> MEELFNALPQPLQQLSLALAGEIPLTDHIFEQAASTWHVQPRSLTYKLLDHIPFATPVVVPPSIYHSLDWSKCFAVNQDRVERIPTIDNPDDVYVPNSDIGPLLTSLHTIPDYGFLHPTIENDATTLRAERARCASTFYKIASSQARQVKLDPIRMLGFLLLVQARPRVPSGLVTDQPTRRDPTLSPALHAIWQVMQYYKVAGVYYAPALVVPSGAIWWIPPPGKRNVVSVQYLLTDLISLAILAHMTDMSPTLELTGVLMYLRAASSHSYAYTLLQMKSVFPALSLRSMYRNKGFGGKAPAIEWTEPRSKYKFRWTGVTQLHDGLRPRSPSMDVPTLETLAKYELVDIGHTIIRERNAHPQHNHDSVRFVRDVMALTSGMYLVRQPTMSVLREYSQVPDIKDPIPPSAWTGPIGNVRYLLPSVQGPARHLYDTWRAAARQIAQDPQWHDPLNQAIMRAQYVTARGGSSASLKFALKVTGIVLPEYDDSKVKKSSKIYQAAQIARIAFMLLIAAIHAEVTMGIRNQVQRRARSIMPLNVIQQAISAPHTLVANYINKHMNLSTTSGSVVTDKVIPLILYASTPPNTVVNVDIKACDASITYNYFLSVICGAMHEGFEVGNADAAFMGVPSTIVSDRRSPVAPYSRPISGLQTMVQHLADLYAAGFRYSVSDAFSSGNKFSFPTSTFPSGSTATSTEHTANNSTMMEYFLNVHAPSHVKSASLKRILTDMTIQRNYVCQGDDGILLLPHEAASKISADDMNELLTCLRDYGQLFGWNYDIDWSDTAEYLKLYALMGCRIPNTSRHPPVGKEYAAPQTDEIWPSLIDIVIGHHLNGVTDVLNWREWLRFSWAFACYSSRGGYTNPRGQSFSAQYPWWTFVYLGIPPILLPGQTPFIHSCYMPPGDQGMFSILNGWRDWLISHASTTLPPLRHNHPVWGLSDVPSLLSQFGVYAGYHAAQHYRRPKPAPETASSDSINQITSDLTEYLFYDSALKARVMKGRYNWERLSSSLSLNVGSRVPSLFDVPGKWVAAGRDAEKPPPSSVEDMFTSLNRCIRRPTHSFSRLLELYLRVHVALGESIPLAIDPDVPQVAGADPANDDHWFKYTCLGDIPSATRNYFGESLFVGRVVSGLDVEAVDATLLRLKILGAPPEAFIAVLNGIGMSDSEAHQIAGRISLANAQLVQIARVVHLSIPSSWMTLNTGPYIHHHAYDFKPGITQPSAKSRDKSIWMSPILKLLCTSYAMTVAGPVRTSIVTEIDGSAAALSGNLRVWMRDV;> MITIVVIPTAHFSWTDTNFLNSVDYRLTSQPKIRDRFAVYAPGWLRRQLDEFSASLTASELLQALQTIPIPVKARCLLLPKPKRFAQWLLDVPSANIWHIPVTTLRATVASKHPSSDVYNYIPDHVPPNAEFDTVTRRVAAGRDIYVRSTKVIGAPLCLAAPAKYYAGYLSTHQLDGIYPENWAPDNFHKREFCLTILPSLLGPRTFLLDVDADRDASYPLSVLWPQLRALALKSRLLLPPVALLRRVVDPGLKPTWSADSDAAFRALRLSRPSSASKPVGFDFSALPVVDIICLLESEPDDHGRIAPGTRLTIHSVPTDLLTSLSIQEGVRYPLRQESGMFVHWVLLALLMSDDVTISGTRRSVKLETAHASARPFVHITVERCASARIIDVRGSPAMYANAVCLTLPKGSYKSTIIDTLPAMFSDLPILEQAAVIDSDALGDSLRPSFETQFLERLENLDPNLLDRAVASILSPTSDTSDDAVTTVLDAFNALYREIMTPAQRARLPLLTQQGRVLAFAHSDYELLSANIPIQVVRGSIPIDHVVNLLARRNRVGGTALQVLLDYCYRTQASPLAPTPAGRLYKQLFGPWLMVPRLSEPLIKLRLVASAPAKVLRAAGWTIDGDPPLEVSCLCAYVTDRAAATALIERRLDSRALVTVGGDQLMFVEYAPPLPLVSIPRTFLLPVTYVVHWVPPQRVLLNGGNVSFTSGLEWTFDDDPQVVTSTGV;>MPRRSARKAQSAIASPADTNVVPAKDAPTTNSPPSTTSPNQAAADANQQQAGIVSSQSGPNAVGDSAPSSSVNNDGDIITRPTSDSIAAVANATKPAAVVSDPQSMKVTPIVNPSSYVCNVCNARFSTMSALSEHLRSDHRDDASTLLATPMINNAIRSFLTAWDDIRILSPDVSSKSLSAYLDSAVANGPELIIEDTGLCTSFMLLDNIPSAHLTKELIGFTWFMQMYQMTPPLPEGAVNRIVC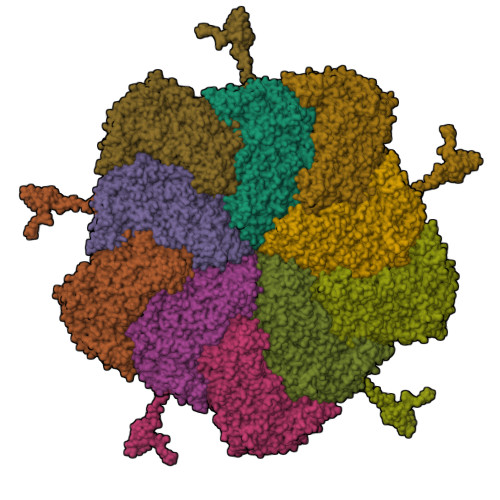MTNWASLGDEGRGLEVRLPPPTDSSVHAYKTVLSRGYIDNAQFNPLALRSNVLLMLLQFTLSNLKINKSSTFTSDVTTITSGRMIRAFEGRPELLALAYPGRAVLPTQTKNAQFLSTAIADRIGRLDRANLIGGEVSAMVECMELCDALTLHIRETYIMLLRSMHQDPTQIVQIVNECANNLLNSTIPISLRPTILCPWFASSEDLRLQQVMHLVNISSNTAAALPLVEALSTLLRSVTPLVLDPTVLTNAITTISESTTQTISPISEILRLLQPMGNDYAAFWKCIASWAYNGLVTTVLSEDAFPDSSQSITHLPSMWKCLFLTLAGPMTSDPHSPVKVFMALANLLAQPEPIAIGVPGMHQTTPASQFSHPGVWPPGFLNPQLINPQQAPLLRAFAEHIRANWPQPSEFGYGSTLQGSANLFIPSNRMVYPWPNQPLPRLTVAPTYDSAMSNWISTTIAFFIRVVNSVNMTATVNDLTRRTMTGVMTAMRQVKTMTPFYIQHMCPTELSVLASVTVTPPFQVPFTRLVQNDVITNVLVARVDPAQRGDAAVDIRATHATFAAALPVDPAAIVVAMLCGQTETNLIPSHHYGKAFAPLFASNAMFTRNQRAVITREAFVCARSAVAQCQDAGFLVPRPLDALRQFDVTSAAAAEIMHAVNDAFKTAFDLDGALLDGLALYGDPRIADLSAAYLQYGGNVVREHVPPGPSHIHRALQQVESTFMAEMNLFNVARGNLYLVQTATNGNWSPMAPVAAPPFVRGGPNVRVVGRFGTIVPRPNGLEPQLIDDGNVPRDIAGDWVYPSDVLQVSVAVFRDYVWPMVKAGRTRVLVELGHYVYTLHYYDPQISLDEAPILEEWLSKINPAGIPPVPFCIPIPQVYPCITARRVHYAFTSENNNDSLFSTNAASIDTAFGENAAVSPLRWPGLVDPNYRVGTNDLPNRITLYNSLYRYNFTYPTLDGIMYVRSAT[10x]>VANTTYKAPIERPEDFLKDKEKAKEWERKEAERIEQKLERSEKEALESYKKDSVEISKYSQTRNYFYDYQIEANSREKEYKELRNAISKNKIDKPMYVYYFESPEKFAFNKVIRTENQNEISLEKFNEFKETIQNKLFKQDGFKDISLYEPGKGDEKPTPLLMHLKLPRNTGMLPYTNTNNVSTLIEQGYSIKIDKIVRIVIDGKHYIKAEASVVSSLDFKDDVSKGDSWGKANYNDWSNKLTPNELADVNDYMRGGYTAINNYLISNGPVNNPNPELDSKITNIENALKREPIPTNLTVY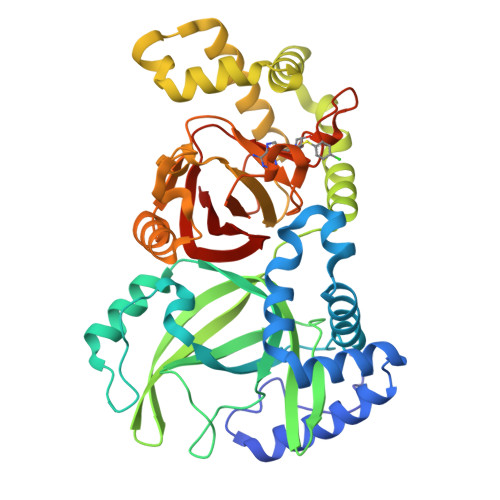RRSGPQEFGLTLTSPEYDFNKLENIDAFKSKWEGQALSYPNFISTSIGSVNMSAFAKRKIVLRITIPKGSPGAYLSAIPGYAGEYEVLLNHGSKFKINKIDSYKDGTITKLIVDATLIP[2x]> MASVHGTTYELLRRQGIDTVFGNPGANELPFLKDFPEDFRYILALQEACVVGIADGYAQASRKPAFINLHSAAGTGNAMGALSNAWNSHSPLIVTAGQQTRAMIGVEALLTNVDAANLPRPLVKWSYEPASAAEVPHAMSRAIHMASMAPQGPVYLSVPYDDWDKDADPQSHHLFDRHVSSSVRLNDQDLDILVKALNSASNPAIVLGPDVDAANANADCVMLAERLKAPVWVAPSAPRCPFPTRHPCFRGLMPAGIAAISQLLEGHDVVLVIGAPVFRYHQYDPGQYLKPGTRLISVTCDPLEAARAPMGDAIVADIGAMASALANLVEESS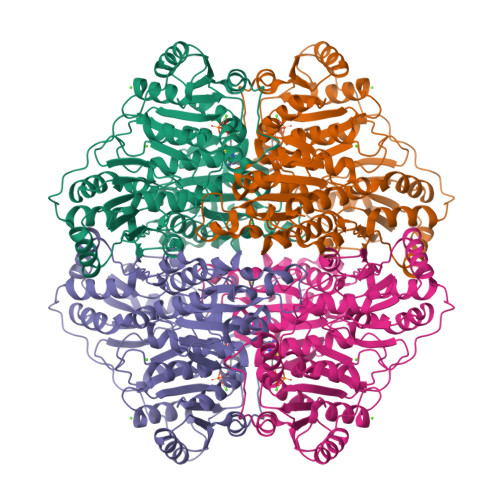RQLPTAAPEPAKVDQDAGRLHPETVFDTLNDMAPENAIYLNESTSTTAQMWQRLNMRNPGSYYFCAAGGLGFALPAAIGVQLAEPERQVIAVIGDGSANYSISALWTAAQYNIPTIFVIMNNGTYGALRWFAGVLEAENVPGLDVPGIDFRALAKGYGVQALKADNLEQLKGSLQEALSAKGPVLIEVSTVSPVK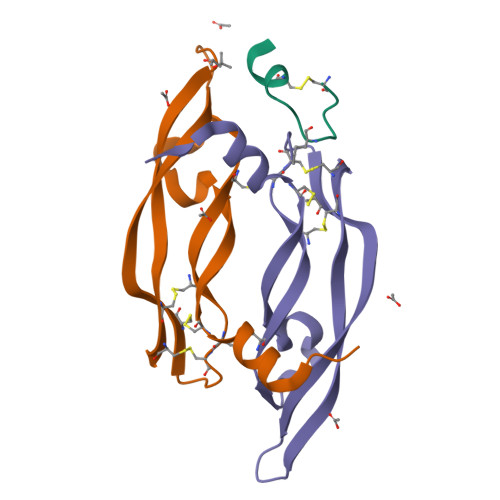> CDIHVLWEWDCFEKLX;>[2x]EVVKFMDVYQRSYCHPIETLVDIFQEYPDEIEYIFKPSCVPLMRCGGCCNDEGLECVPTEESNITMQIMRIKPHQGQHIGEMSFLQHNKCECRPK>[2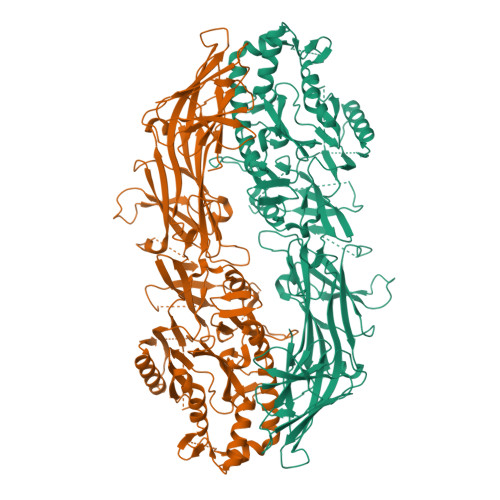x]MSLQRIVRVSLEHPTSAVCVAGVETLVDIYGSVPEGTEMFEVYGTPGVDIYISPNMERGRERADTRRWRFDATLEIIVVMNSPSNDLNDSHVQISYHSSHEPLPLAYAVLYLTCVDISLDCDLNCEGRQDRNFVDKRQWVWGPSGYGGILLVNCDRDDPSCDVQDNCDQHVHCLQDLEDMSVMVLRTQGPAALFDDHKLVLHTSSYDAKRAQVFHICGPEDVCEAYRHVLGQDKVSYEVPRLHGDEERFFVEGLSFPDAGFTGLISFHVTLLDDSNEDFSASPIFTDTVVFRVAPWIMTPSTLPPLEVYVCRVRNNTCFVDAVAELARKAGCKLTICPQAENRNDRWIQDEMELGYVQAPHKTLPVVFDSPRNGELQDFPYKRILGPDFGYVTREPRDRSVSGLDSFGNLEVSPPVVANGKEYPLGRILIGGNLPGSSGRRVTQVVRDFLHAQKVQPPVELFVDWLAVGHVDEFLSFVPAPDGKGFRMLLASPGACFKLFQEKQKCGHGRALLFQGVVDDEQVKTISINQVLSNKDLINYNKFVQSCIDWNREVLKRELGLAECDIIDIPQLFKTERKKATAFFPDLVNMLVLGKHLGIPKPFGPIINGCCCLEEKVRSLLEPLGLHCTFIDDFTPYHMLHGEVHCGTNVCRKPFSFKWWNMVP>[2x]GMPPVWTLPRLYQHFQGAIDLELWTIPYYLTVLYSIKDPTTVPYRLIQAAVYQEMLHAQLVSNIANAYGYSPTLSAPEYVGTAVPHIDFDLDTPNPTSIFTPYSAELGPLDLTRVNTMCLIEYPEWRTQREPDLADDVTDYGSIGEFYDALRVGMEQLRGHVRGNQKQMDEFGPFYQNSPPLTVTESGDAGFLQALTLVDIIVDQGEGQTQPVETIPTEFQNTADGFQ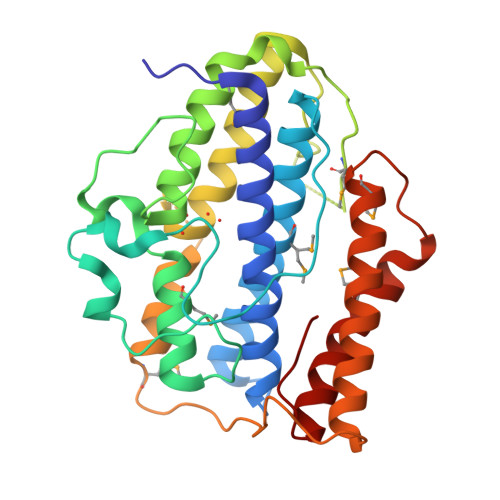DAWPHFQRFDFIRRMPNWPGVYTGVTDPPAGSPGAEAQARLIADFAGFLDILNGMFSGGGAPPAFGVQMAKLGGDILSCWKLGAVPRYS>QGHMATNVTYQAHHVSRNKRGQVVGTRGGFRGCTVWLTGLSGAGKTTVSMALEEYLVCHGIPCYTLDGDNIRQGLNKNLGFSPEDREENVRRIAEVAKLFADAGLVCITSFISPYTQDRNNARQIHEGASLPFFEVFVDAPLHVCEQR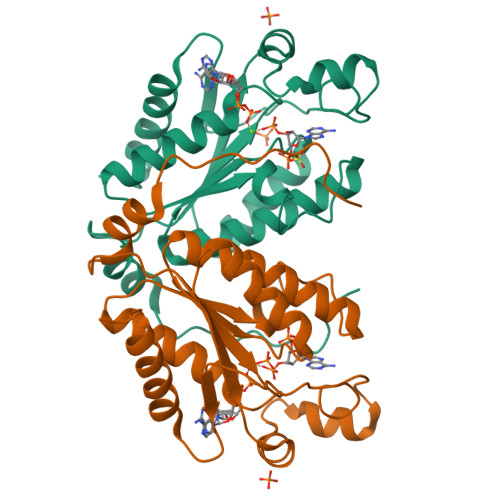DVKGLYKKARAGEIKGFTGIDSEYEKPEAPELVLKTDSCDVNDCVQQVVELLQERDIVP[2x]>MSEIVVSKFGGTSVADFDAMNRSADIVLSDANVRLVVLSASAGITNLLVALAEGLEPGERFEKLDAIRNIQFAILERLRYPNVIREEIERLLENITVLAEAAALATSPALTDELVSHGELMSTLLFVEILRERDVQAQWFDVRKVMRTNDRFGRAEPDIAALAELAALQLLPRLNEGLVITQGFIGSENKGRTTTLGRGGSDYTAALLAEALHASRVDIWTDVPGIYTTDPRVVSAAKRIDEIAFAEAAEMATFGAKVLHPATLLPAVRSDIPVFVGSSKDPRAGGTLVCNKTENPPLFRALALRRNQTLLTLHSLNMLHSRGFLAEVFGILARHNISVDLITTSEVSVALTLDTTGSTSTGDTLLTQSLLMELSALC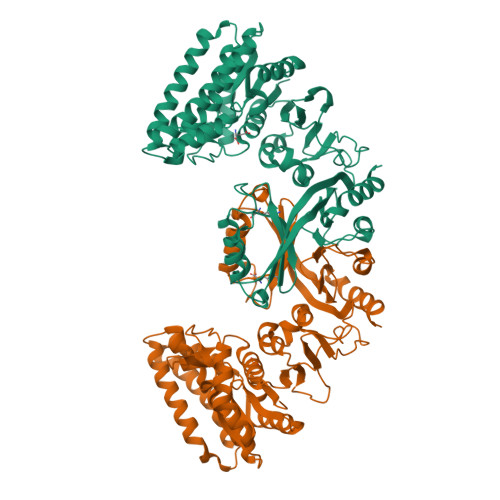RVEVEEGLALVALIGNDLSKACGVGKEVFGVLEPFNIRMICYGASSHNLCFLVPGEDAEQVVQKLHSNLFE[2x]>MHHHHHHPTTQPRLSFLAVPTEDNAHEGVKKLWSKAEANMGFVPNVFRAQALNGEQFLAWWNYFNLLVNKEGGLSNAERELLAVVVSGLNRCVYCAVSHGAALREFSGDAVKADAVAVNWRQAELSEREQAMCAYAEKLTLRPAEMTEADLAPLRAAGLSDEAILEAVQVIAM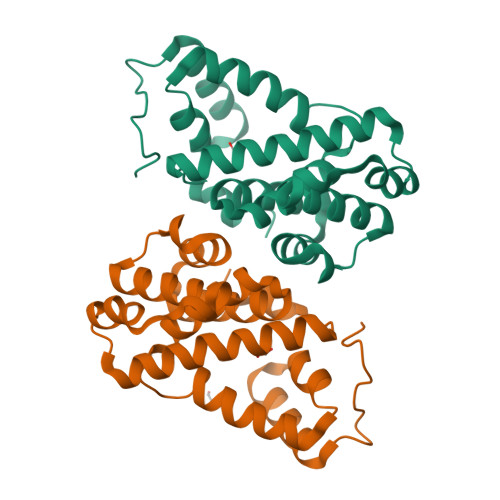FNMTNRVSSALGFVPNPEYHIQSR[12x]> MSAEVIGQVEEALDTDEKEMLLFLCRDVAIDVVPPNVRDLLDILRERGKLSVGDLAELLYRVRRFDLLKRILKMDRKAVETHLLRNPHLVSDYRVLMAEIGEDLDKSDVSS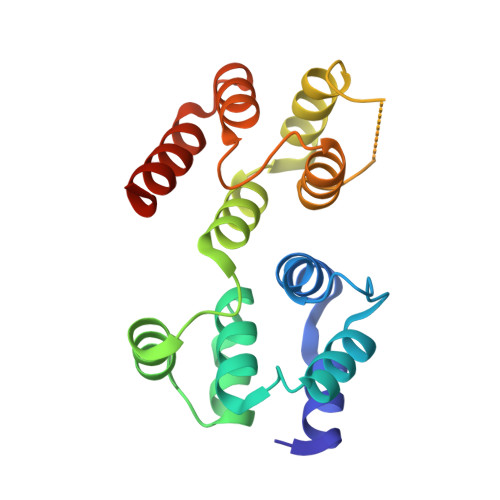LIFLMKDYMGRGKISKEKSFLDLVVELEKLNLVAPDQLDLLEKCLKNIHRIDLKTKIQKYKQSVQGAGTS> ATVRT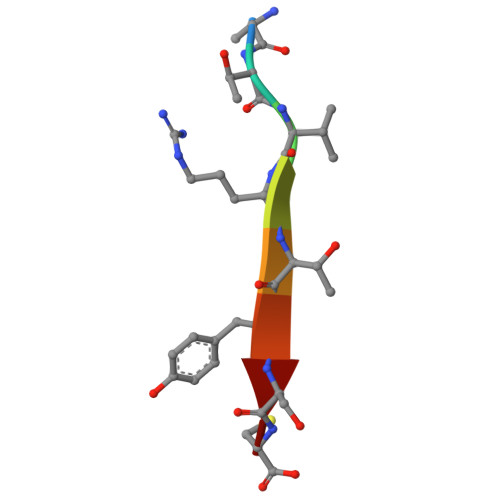YSC> TG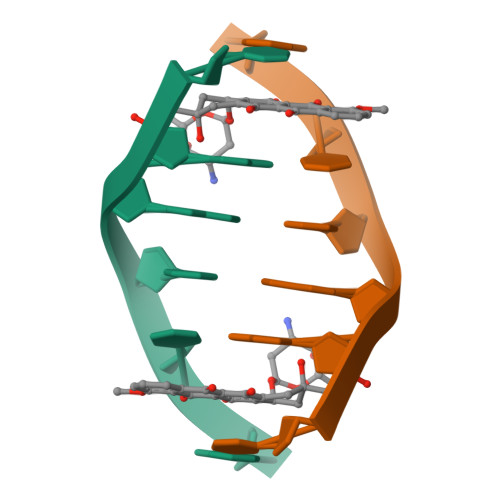GCCA> GSHMRIALMQHTARPLDPQHNLDLIDDAAARASEQGAQLLLTPELFGFGYVPSQICAQVSAEQVDAARSRLRGIARDRGIALVWSLPGPEGPEQRGITAELADEHGEVLASYQKVQLYGPEEKAAFVPGEQPPPVLSWGGRQLSLLVCYDVEFPEMVRAAAARGAQLVLVPTALAGDETSVPGILLPARAVENGITLAYANHCGPEGGLVFDGGSVVVGPAGQPLGELGVEP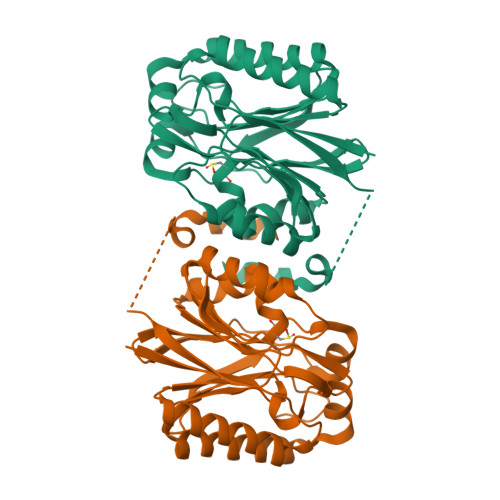GLLVVDLPDQSQDAGSDSADYLQDRRAELHRNWL>AMGKYVKVQDFYDQLGKYVLVAPGKFSGTVAATDLSTGWTMAWLAAWNYGDTCPIMHHMAAFPSPDPYKEFEFVVNTQGGKNLFIYGVPVTVEDPGEGMKIYRIKYDGTRMNLQRDAAEVSGLGLGVHVTITPEADGYAVGDGQKDICAEFDRETDMVRYAWAFDWDPNVKDLKRAWLDGGTMTIKRLKPTLPGGRYDLQGSKGNKIDWELVPGGELAIEDGKVSGDRPLHSVANDALVFDPRGKWAVASMRLPGVCVVFD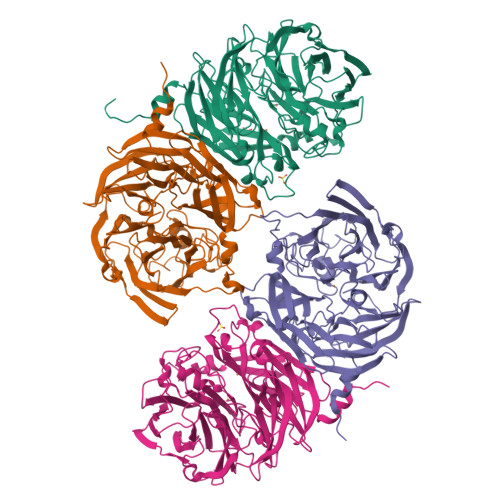RENQVPVAVLAGPKGTPSQFQLVKVDDDTWTVDIPEVISAGHQAGFSPDGQSFLFMNSLRQNNIMVWDSSNHDDPTTWEKKAVVESPDWRGAYPNTFHMVFTPDAKKIYVTMWWPSPTPNGIAVIDAVNWEVLKEVDLGPDMQTLAITYDGKFVVGTLSGYQNTASAIVVMETETDEVLGFLPSPMGHHDNVIVPRTLEDLRISRSTTT[4x]>MAAGFGRCCRVLRSISRFHWRSQHTKANRQREPGLGFSFEFTEQQKEFQATARKFAREEIIPVAAEYDKTGEYPVPLIRRAWELGLMNTHIPENCGGLGLGTFDACLISEELAYGCTGVQTAIEGNSLGQMPIIIAGNDQQKKKYLGRMTEEPLMCAYCVTEPGAGSDVAGIKTKAEKKGDEYIINGQKMWITNGGKANWYFLLARSDPDPKAPANKAFTGFIVEADTPGIQIGRKELNMGQRCSDTRGIVFEDVKVPKENVLIGDGAGFKVAMGAFDKTRPVVAAGAVGLAQRALDEATKYALERKTFGKLLVEHQAISFMLAEMAMKVELARMSYQRAAWEVDSGRRNTYYASIAKAFAGDIANQLATDAVQILGGNGFNTEYPVEKLMRDAKIYQIYEGTSQIQRLIVAREHIDKYKN[4x];> MFRAAAPGQLRRAASLLRFQSTLVIAEHANDSLAPITLNTITAATRLGGEVSCLVAGTKCDKVAQDLCKVAGIAKVLVAQHDVYKGLLPEELTPLILATQKQFNYTHICAGASAFGKNLLPRVAAKLEVAPISDIIAIKSPDTFVRTIYAGNALCTVKCDEKVKVFSVRGT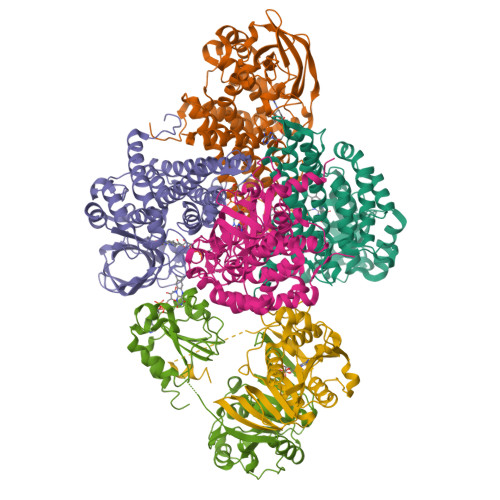SFDAAATSGGSASSEKASSTSPVEISEWLDQKLTKSDRPELTGAKVVVSGGRGLKSGENFKLLYDLADQLHAAVGASRAAVDAGFVPNDMQVGQTGKIVAPELYIAVGISGAIQHLAGMKDSKTIVAINKDPEAPIFQVADYGIVADLFKVVPEMTEILKKK;> MAELRVLVAVKRVIDYAVKIRVKPDRTGVVTDGVKHSMNPFCEIAVEEAVRLKEKKLVKEVIAVSCGPAQCQETIRTALAMGADRGIHVEVPPAEAERLGPLQVARVLAKLAEKEKVDLVLLGKQAIDDDCNQTGQMTAGFLDWPQGTFASQVTLEGDKLKVERAIDGGLETLRLKLPAVVTADLRLNEPRYATLPNIMKAKKKKIEVIKPGDLGVDLTSKLSVISVEDPPQRTAGVKVETTEDLVAKLKEIGRI(2S)-(4-{3-[(4,5-dichloro-1-methyl-1H-indole-2-carbonyl)amino]oxetan-3-yl}phenyl)(pyridin-3-yl)acetic 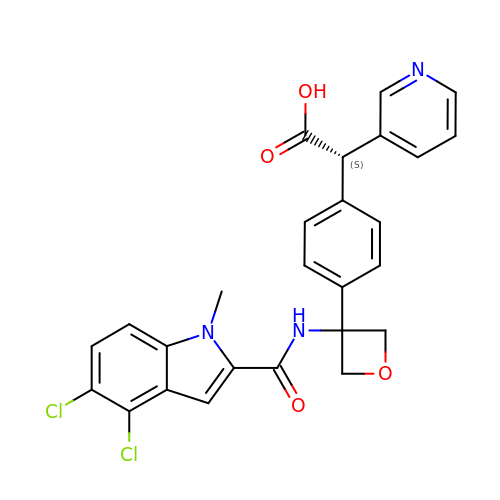acid | C26 H21 Cl2 N3 O4 | LHTXTAIWLHZCIX-QFIPXVFZSA-N>EWTGDNTNAYYSDEVISELHVGQIDTSPYFCIKTVKANGSGTPVVACAVSKQSIWAPSFKELLD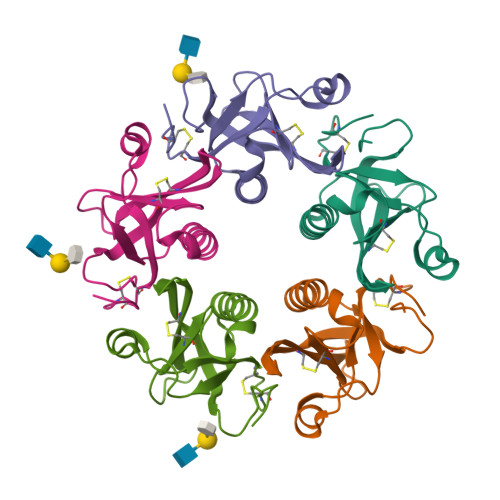QARYFYSTGQSVRIHVQKNIWTYPLFVNTFSANALVGLSSCSATQCFGPK[5x]> MGPPEKDSKAILKARGLEEEQKSESTMSPSENVSRAILKDSGSEEVEQASERKMTSPENDSKSIQKDQGPEQEQTSETLQSKEEDEVTEADKDNGGDLQDYKAHVIAKFDTSVDLHYDSPEMKLLSDAFKPYQKTFQPHTIILHGRPGVGKSALARSIVLGWAQGKLFQKMSFVIFFSVREIKWTEKSSLAQLIAKECPDSWDLVTKIMSQPERLLFVIDGLDDMDSVLQHDDMTLSRDWKDEQPIYILMYSLLRKALLPQSFLIITTRNTGLEKLKSMVVSPLYILVEGLSASRRSQLVLENISNESDRIQVFHSLIENHQLFDQCQAPSVCSLVCEALQLQKKLGKRCTLPCQTLTGLYATLVFHQLTLKRPSQSALSQEEQITLVGLCMMAAEGVWTMRSVFYDDDLKNYSLKESEILALFHMNILLQVGHNSEQCYVFSHLSLQDFFAALYYVLEGLEEWNQHFCFIENQRSIMEVKRTDDTRLLGMKRFLFGLMNKDILKTLEVLFEYPVIPTVEQKLQHWVSLIAQQVNGTSPMDTLDAFYCLFESQDEEFVGGALKRFQEVWLLINQKMDLKVSSYCLKHCQNLKAIRVDIRDLLSVDNTLELCPVVTVQETQCKPLLMEWWGNFCSVLGSLRNLKELDLGDSILSQRAMKILCLELRNQSCRIQKLTFKSAEVVSGLKHLWKLLFSNQNLKYLNLGNTPMKDDDMKLACEALKHPKCSVETLRLDSCELTIIGYEMISTLLISTTRLKCLSLAKNRVGVKSMISLGNALSSSMCLLQKLILDNCGLTPASCHLLVSALFSNQNLTHLCLSNNSLGTEGVQQLCQFLRNPECALQRLILNHCNIVDDAYGFLAMRLANNTKLTHLSLTMNPVGDGAMKLLCEALKEPTCYLQELELVDCQLTQNCCEDLACMITTTKHLKSLDLGNNALGDKGVITLCEGLKQSSSSLRRLGLGACKLTSNCCEALSLAISCNPHLNSLNLVKNDFSTSGMLKLCSAFQCPVSNLGIIGLWKQEYYARVRRQLEEVEFVKPHVVIDGDWYASDEDDRNWWKN;> MTSHRQS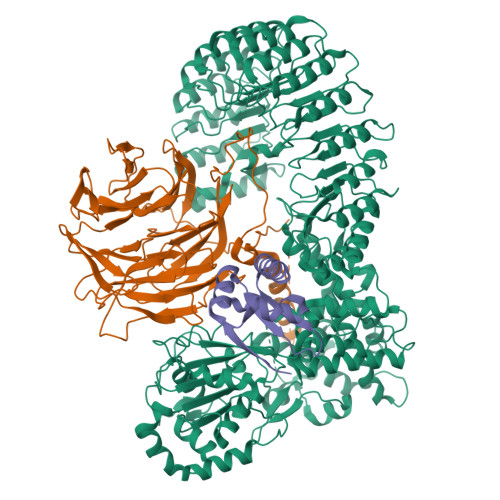SDTFGGILPSTLSSRYLSIVNQLPEEFSSVVSEMMVHLENIFSLAENFFQAIERFSRTPDLLERNKMSIGVGAEGDSWPCHVSHEAPMGSAQTTENSAKEEDKQVPESAALQHPKFKSTPGPQLPTRRRFLSESDELQDPQPVWDAEPQFCQGFLIQGLWELFMDSRQKNQQEHGGEDSSQESKDSGLCDFKPEPQPRHRNSLSDSADPFLIKSPSALLDYYQEDVSRPQPETQESSGRADKFLKPLSWGSEVLESSCNQPSTALWQLERFTVPQALQKVRVLKHQELLLVVAVSSFTRHVFTCSQSGIKVWNLVNQVAEDRDPESHLKCSVQDNKVYLRTCLLSSNSRTLFAGGYNLPGVIVWDLAAPSLYEKCQLPCEGLSCQALANTKENMALAGFTDGTVRIWDLRTQEIVRNLKGPTNSARNLVVKDDNIWTGGLDACLRCWDLRMAKVSLEHLFQSQIMSLAHSPTEDWLLLGLANGQHCLFNSRKRDQVLTVDTKDNTILGLKFSPNGKWWASVGMGNFITVHSMPTGAKLFQVPEVGPVRCFDMTENGRLIITGSRDCASVYHIKY;> MASHTADADAKPDSDSQKLLNVLPVSLRLRTRPWWFPIQEVSNPLVLYMEAWVAERVIGTDQAEISEIEWMCQALLTVDSVNSGNLAEITIFGQPSAQTRMKNILLNMAAWHKENELQRAVKVKEVEEFLKIRASSILSKLSKKGLKLAGFPLPLEGRETQMES>[10x]MASHAEKPLVGSVAPDFKAQAVFDQEFQEITLSKYRGKYVVLFFYPLDFTFVCPTEITAFSDR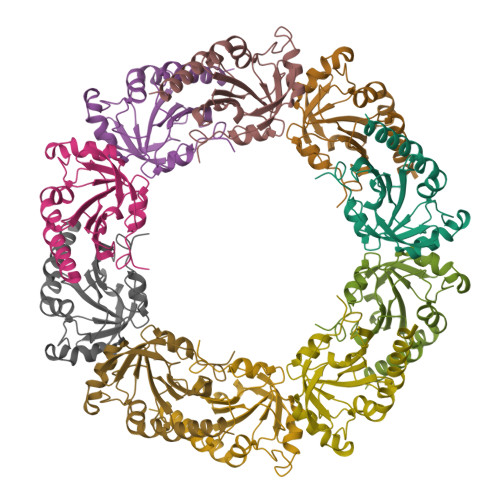YKEFKDINTEVLGVSVDSQFTHLAWIQTDRKEGGLGDLAYPLVADLKKEISKAYGVLTEDGISLRGLFIIDKEGVVQHATINNLAFGRSVDETKRVLQAIQYVQSNPDEVSPAGWKPGDKTMKPDPKGSKEYFSAVQDPNSSSVDKLAAALEHHHHHH>HHHHHHMNSSIVSQHFFISLKSSLDLQCWKSSSPSSISMGEFKGIHDKLQILKLPLTMSDRGLSKISCSLSLQTEKLRYDNDDNDDLELHEELIPKHIALIMDGNRRWAKAKGLEVYEGHKLIIPKLKEICDISSKLGIQVITAFAFSTENWKRSKEEVDFLMQLFEEFFNEFLRFGVRVSVIGCKSNLPMTLQKCIALTEETTKGNKGLHLVIALNYGGYYDILQATKSIVNKAMNGLLDVEDINKNLFEQELESKCPNPDLLIRTGGEQRVSNFLLWQLAYTEFYFTNTLFPDFGE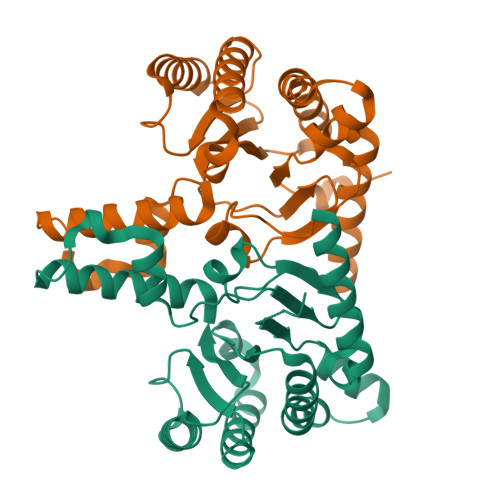KDLKKAILNFQQRHRRFGGHTY[2x]>[2x]APQPPNILLLLMDDMGWGDLGVYGEPSRETPNLDRMAAE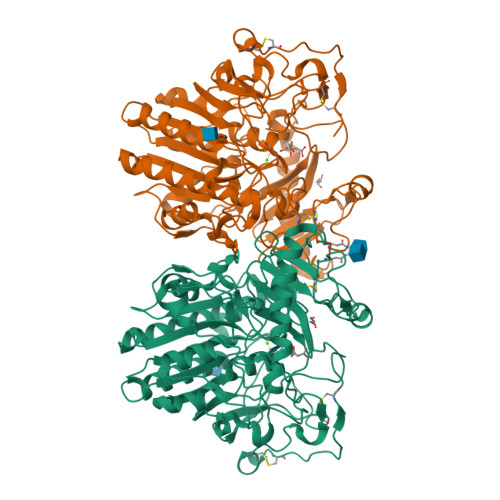GLLFPNFYSANPLASPSRAALLTGRLPIRNGFYTTNAHARNAYTPQEIVGGIPDSEQLLPELLKKAGYVSKIVGKWHLGHRPQFHPLKHGFDEWFGSPNCHFGPYDNKARPNIPVYRDWEMVGRYYEEFPINLKTGEANLTQIYLQEALDFIKRQARHHPFFLYWAVDATHAPVYASKPFLGTSQRGRYGDAVREIDDSIGKILELLQDLHVADNTFVFFTSDNGAALISAPEQGGSNGPFLCGKQTTFEGGMREPALAWWPGHVTAGQVSHQLGSIMDLFTTSLALAGLTPPSDRAIDGLNLLPTLLQGRLMDRPIFYYRGDTLMAATLGQHKAHFWTWTNSWENFRQGIDFCPGQNVSGVTTHNLEDHTKLPLIFHLGRDPGERFPLSFASAEYQEALSRITSVVQQHQEALVPAQPQLNVCNWAVMNWAPPGCEKLGKCLTPPESIPKKCLWSHHHHHHH>[4x]MSKPQNNDTLELDDILSQPVKDKERFAAFMMRKLAENKPAQNDNLFGNFKLDFDLDFEVPLIKKSQAKPKSKLPEVQPLGELVSKNSAATEKVNEPPVDQAPNENVPPRRSPTLSPNNRRSMRRSGNVPGSDKLRRHAIRRRSRSCGRQLLPEFEETVNLTRSISSPVNFLPEISSTPCTEKQKEEVAKNTTRVETDKPAEKPMELSQEPEPENPLQTKVTSPARNPILAAEIEQICKERQSSFHKNVLQLDYSGRAPYSRPPTPSSPSVAGLRRTYTMEKGPAPGQLLLSPSHRYDTPSKMPVVKAKRFNQELMVPDTPERQSHDPAWQSEPQPEFVVPETQPQDLGELVQTLSRSAISPIVVINTSNSNRSVRRDAVAMKSVPTSPVTALSSPPIAPSPRRSAAASPQKSIAQLPRVEENMDAIMTDDESDEHPSTVPLNLAPSGGNTTRQRRLRSSNRARATIESQESSMRLLNLHKSVNAKKSKPRKTAIPLNKAPSAPINGEQFARELTRMSNYEILDLRKRNSLNEIYPLNGHRNHRSEKLILEEEIQRELLRRNLMDEAEGLPKQQSSDDSNEDYIPVPPKTQSLRTKSNDRSQGRGRPRSTRRDLPMTTELVNYLGLSQTLETRRKSSKDGKRCLYTKGSSDHEDNDSLSPVKLPRLSKSIQIVPPPPVSLRYSQSLQNLPCSGKFDFDNVVMAAPPDFHDSVNSDAIEIAPPPPEYVVNTRGRSTSGRKSNKNDLVLPPPGYEGGQEEEHDERPSQPRCTAKELQQSTQNGRRAMENELVPPPIEYVEEENRNNEQSRRSTKNGNLVDRNTHNAVEYCEPPEPPEYDDSDHGQASILRRSGKKLQHSKQSVQKSNKEQIIAPSYENNEDYDSDEEPIYNEEYGKEESQNKNVTRRKSDKDEMASHTLECIEGPDPNWNSSCNKQNRNHQNASKSKENDKLANRSSKSQKLSNPRQNAVGTEKSVALSNRGEECTEKSSDVMESLRVNTPTPPIDQNSDDVPSRNPSPSRTLLSDDVPSTSRAALEFLQRSQNMSKSRPPDESSADVVFKKPLAPAPRAKSKKGKSEVDKLKLAKMPVEAEELNTTGIRRSKRGQVPLQMSWCHTMDPSKFNFMSGFIEPRSKNSKTKKGNLSKAKKASATKPKPTVEKNLPDNRGPLCSSTPRISEKLPGAIPHSESLGLSTLTWEETEVQAEAEKVPKKRGRPKKAVGGVQTDTEAEPEPEPEPMISSVAPLTSDQEEPDVPDEQAPYTEAALGPVVFSTPLRDEQEEASTKLMQWLRGVGDAPPSASMSDENASVSSANELIFYQVDGIDYAFYNTKEKAMLGYM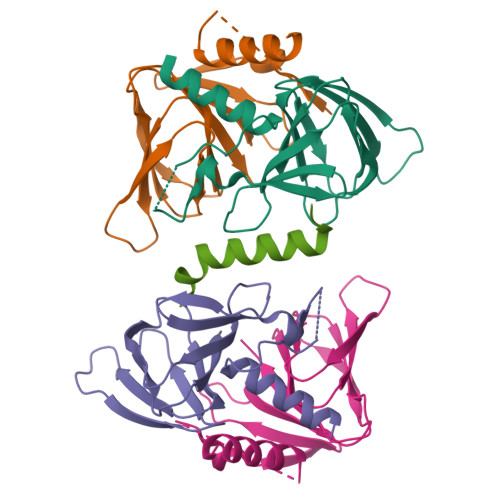RFKPYQKRSMKQAKVHPLKLLVQFGEFNVETLAVGEEKEVHSVLRVGDMIEIDRGTRYSIQNAIDKVSVLMCIRS;> MANAVVDEETLEAMVYERSKAWSSKMADFASLEDGMEIDVAEFDNLFHGEDEDPDLDDVAKEAVEDNVPDEAKLEMGHINATSVTELTLILCANEDNEAKAEIEEILNQTVPVVEEHKRKWREAGLDRILDTFDEKQIEHHVGRWMRRHNSVYLEASPPKYLPPHHNSISDESDESMHSIDTARYIQQSRRRNAHMTNKNMTTIKMYRKHSHKRDELRAKYAYGDEQEHRHHMQAVLLRRRERERQLAYLASTPMQCVYSSGHHMRRKNLRKRRINSWMFDSASSSEEDTSFGGCDCHSCRRHYALSRSVYQSCPYGRGQREYHHRQMASRTMHTMRRQHTFDMEMDLRPRLPENECSCCNSDRLCSNVIHIANSSTEEWVVENRSNHLTQETQEKTRKQKHQPMDARKVSHQPVCSKGHEQKPLSSKATSVSKLVLSKEKYMQMFDSESSDEDNALAKKGLLCCSDKKKGMTFPTPNAAGKITHPTSSAKKAIRKEARPNGLAQIQEEGPTATNSPIESTYLPVAHMKSVSIDGSSGTSATFESPAKKAPKRGIRETSPLNGNELQQLISTIPIADEKASSLMEKVDNCIGRESFDDRNKDFMHMENSSTKTAVEKSTKQKRVSGKKSEIPKSIITNNEILEKNSTETLSEKQVAAKAKKQSVRKTGATGKPSTSRLKKSEKTKTTSSVTSTSKLEQVREEESDVSSEVLAKPKPQCSTTASILKQGGDGASNSEDDLQIALAMSKATYKEEQQKRKKTKREPSNKQPQSPAEKSMTVFNNQSVACNSTALANDTACYRVLPKRRGVKRAAAVSTTEEKTATNSSSSPTSSLEEMGSPTGGDPDCTVVTSTTGCEPPASERQEIPATIKITKRGILLHSPSAPEGASFTLTEQGLGKIIGERWARKYLKYHIGSRSFDSRHSVYYQPTPQLAAALSAPQDAQNIGNISGSSASDDDIFEQINRYGTVYSILENNSGDK>GGGHMAIEFDIQESKILKGVYIITPNKFRDLRGEIWTAFTDEYLSKLVPDGIKFKHDKFINSHFNVLRGIHGDVKTYKLVTCVYGEVHQVVVDCRKDSPTYLKWEKFIISYKNQQLILLPPNMGNSHYVS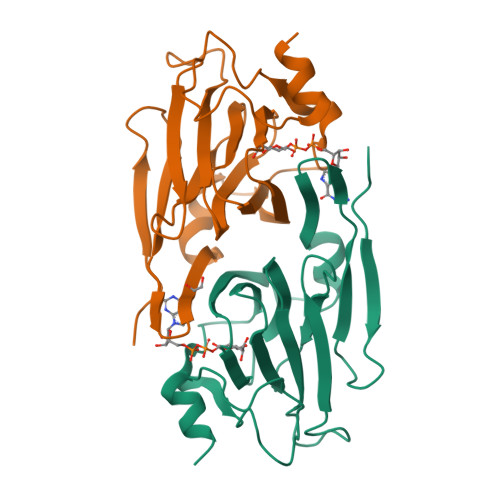SAAAVYYYKLAYEGEYMDAPDQFTYAWNDERIGIDWPTNTPILSDRDILATKNKG[6x]> GLPTMLTPGSSQFLTSDDFQSPCALPNFDVTPPIHIPGEVFNMMELAEIDSMIPMNSVTGKANTMEMYPIPLDDKGSATPIFSISLSPASDKRLQYTMLGEILNYYTHWTGSLRFTFLFCGSMMATGKILLSYS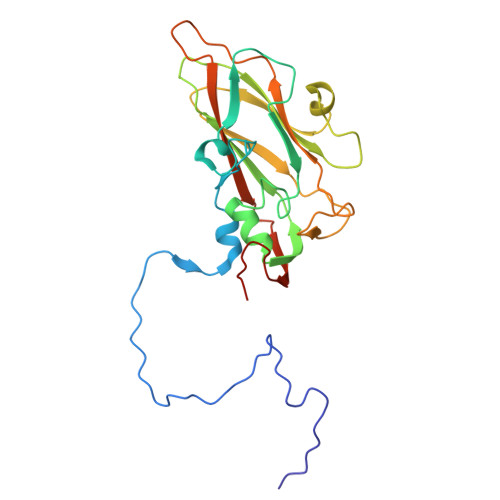PPGAKPPTTRKDAMLGTHIIWDLGLQSSCTMLAPWISNTVYRRCIKDDFTEGGYITCFYQTRIVVPSGTPTSMFMLAFVSACPDFSVRLLRDTNHISQRTLFARAQ> MDKGKSVKSTEKSVGMPPKTPKTDNNAHVDNEFLILQVNDAVFPIGSYTHSFGLETYIQQKKVTNKESALEYLKANLSSQFLYTEMLSLKLTYESALQQDLKKILGVEEVIMLSTSPMELRLANQKLGNRFIKTLQ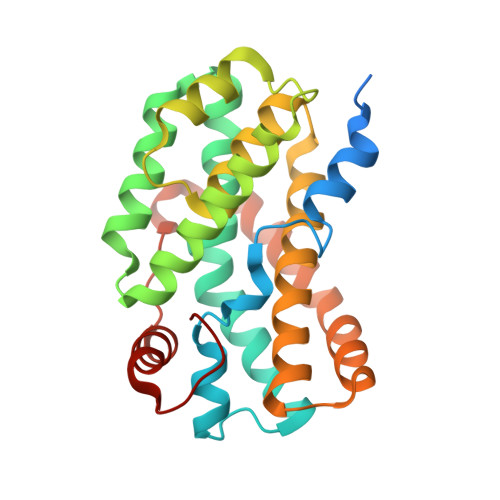AMNELDMGEFFNAYAQKTKDPTHATSYGVFAASLGIELKKALRHYLYAQTSNMVINCVKSVPLSQNDGQKILLSLQSPFNQLIEKTLELDESHLCTASVQNDIKAMQHESLYSRLYMS>[25x]GDNQDRTVANTQPSGPSNSTEIPALTAVETGHTSQVDPSDTIQTRHVVNFHSRSESTIENFMGRAACVFMDQYKINGEETSTDRFAVWTINIREMAQLRRKCEMFTYMRFDIEMTMVITSCQDQGTILDQDMPVLTHQIMYVPPGGPIPAKVDGYEWQTSTNPSVFWTEGNAPPRISIPFISVGNAYSSFYDGWSHFTQDGTYGYTTLNAMGKLYIRHVNRSSPHQITSTIRVYFKPKHIKAWVPRPPRLCPYINKRDVNFVVTEITDSRTSITDTPHPEHSVLATH;>[25x]SPSAEECGYSDRVRSMTLGNSTITTQESANVVVGYGEWPSYLSDREATAEDQPTQPDVATCRFYTLESVQWEKTSPGWWWKFPEALKNMGLFGQNMHYHYLGRAGYTIHVQCNASKFHQGCLLVVCVPEAEMGCADTDTTFPATELTTEDTPHVFTSDSITGKKVQAAVCNAGMGVGVGNLTIFPHQWINLRTNNSATIVIPYINSVPMDNMFRHYNFTLMIIPFAPLNFTDGATAYVPITVTIAPMYAEYNGLRLASTQ;>[25x]GVPVLNTPGSNQFLTSDDYQSPSAMPQFDETPEMHIPGEVRNLMEIAEVDSVVPVNNVTGKTKSMDAYQIPVGTGNTDKTKPIFSFQMDPGYSSVLKRTLLGEMLNYYAHWSGSVKLTFLFCGSAMATGKLLISYSPPGASVPTSRKDAMLGTHIVWDIGLQSSCVLCVPWISQSHYRMVQQDPYTSAGYITCWYQTNIVVPPGAPTSCDVLCFASACNDFSVRLLRDTPFMAQPGKLQ

Viruses from the family Picornaviridae form non-enveloped icosahedral virions that are about 30 nm in diameter. The capsid proteins VP1, VP2, VP3, and VP4 originating from a single polyprotein form a protomer, the basic building block of the icosahedral capsid. The entire capsid consists of 60 such protomers, arranged in 12 pentamer units. Here we show that the exit of the RNA from the particles of echoviruses 18 and 30 requires capsid opening and results in a loss of up to three adjacent capsid protein pentamers.

Specifically, we performed cryo-EM of echovirus 18 virions exposed to pH 6.0 for 10 min, mimicking the acidic environment that the virus encounters in endosomes. Asymmetric reconstruction combined with 3D classification identified subpopulations of echovirus 18 particles that lacked up to three pentamers of capsid protein protomers. We call the particles lacking one or several pentamers open particles. The missing pentamers always formed a single compact opening through the capsid. Reconstructions of the open particles missing one, two, or three pentamers with imposed five-fold, two-fold, and three-fold symmetries, respectively, were determined to resolutions of 3.8, 4.1, and 3.7 Å, which allowed their molecular structures to be built. Except for the missing pentamers, the open particles are similar in structure to that of the activated echovirus 18 particle: increased diameter relative to the native virus, reduced inter-pentamer contacts, absence of VP4 subunits, and holes along icosahedral two-fold symmetry axes. The capsid proteins next to the missing pentamers are more mobile than the rest of the capsid, as indicated by the three times higher temperature factors than the remainder of the capsid. Residues 1–42 from the N termini of VP1 subunits, which were previously shown to interact with membranes and facilitate enterovirus genome delivery into the cytoplasm, are not resolved in the electron density map, indicating that their structures differ among particles. The N-termini of some of the VP1 subunits could reach out of the capsid through the openings formed by the missing pentamers. The openings formed by the removal of one or more pentamers are sufficiently large to allow release of the viral RNA, even if the genome contains double-stranded RNA segments.> MDNYFTAITLLGLRDQNLPPFKDARLQRYKSIKKMIDLIETTTKLAPPMPVELFMLNPTDPEWDDDMTYPTITHATALYKSSALAGNLFLYAYNYNNFTANIRLRTMRY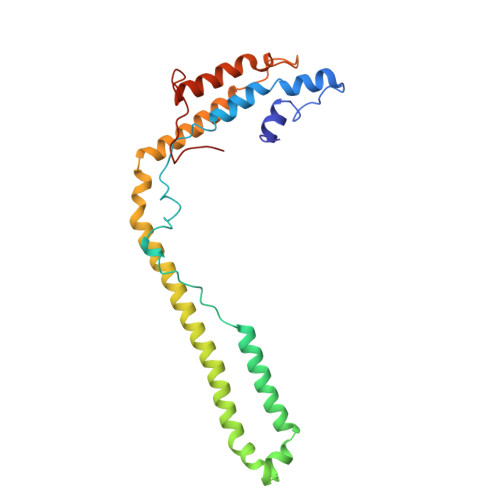LFPVVSLAIFGNIYWDYRSQLVKVNLFDEYIQARAQELVKQNEYLLEHEDVKRYVWWYEDLKETLARVHRQANNHKACDFKDSEIILQDFIRRYTNPKDNLPIKFHPQGQTF> RPLSDQEKRKQISVRGLAGVENVTELKKNFNRHLHFTLVKDRNVATPRDYYFALAHTVRDHLVGRWIRTQQHYYEKDPKRIYYLSLEFYMGRTLQNTMVNLALENACDEATYQLGLDMEELEEIEEDAGLGNGGLGRLAACFLDSMATLGLAAYGYGIRYEFGIFNQKICGGWQMEEADDWLRYGNPWEKARPEFTLPVHFYGRVEHTSQGAKWVDTQVVLAMPYDTPVPGYRNNVVNTMRLWSAKAPNDFNLKDFNVGGYIQAVLDRNLAENISRVLYPNDNFFEGKELRLKQEYFVVAATLQDIIRRFKSSKFGCRDPVRTNFDAFPDKVAIQLNDTHPSLAIPELMRVLVDLERLDWDKAWEVTVKTCAYTNHTVLPEALERWPVHLLETLLPRHLQIIYEINQRFLNRVAAAFPGDVDRLRRMSLVEEGAVKRINMAHLCIAGSHAVNGVARIHSEILKKTIFKDFYELEPHKFQNKTNGITPRRWLVLCNPGLAEIIAERIGEEYISDLDQLRKLLSYVDDEAFIRDVAKVKQENKLKFAAYLEREYKVHINPNSLFDVQVKRIHEYKRQLLNCLHVITLYNRIKKEPNKFVVPRTVMIGGKAAPGYHMAKMIIKLITAIGDVV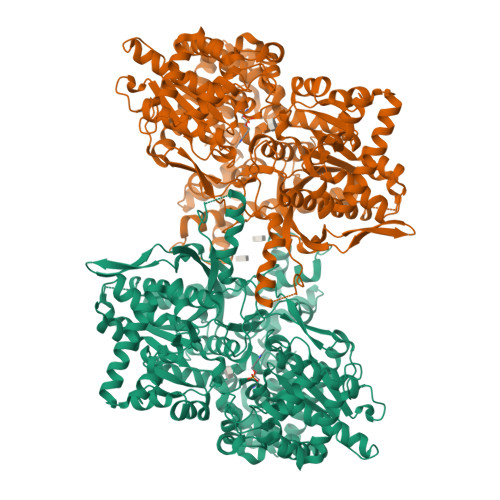NHDPVVGDRLRVIFLENYRVSLAEKVIPAADLSEQISTAGTEASGTGNMKFMLNGALTIGTMDGANVEMAEEAGEENFFIFGMRVEDVDRLDQRGYNAQEYYDRIPELRQIIEQLSSGFFSPKQPDLFKDIVNMLMHHDRFKVFADYEEYVKCQERVSALYKNPREWTRMVIRNIATSGKFSSDRTIAQYAREIWGVEPSRQRLPAPDEKIP>VLRKLKSGLERGLDTFDSTIEIIMQNLKTELESRCSDEVVEQQETENFLEQLISRIFQVVSRLTGVRIRNVQVPDITMEATSENSANVLIPITADVTVSLPFLGEIVDLDLNVDLQTTVSIETDTEDPQVVVGECTNNPESISLTVLHSRFGLVNDVVDIGVNLARRVVSSVVEGELCPRFRELLESLDAECVEKLIGESQ[2x]

Further investigation of BSP30 revealed that it is a mixture of two closely related proteins—BSP30a and BSP30b, sharing 83% amino acid identity, with expression restricted to salivary tissue. Notably, BSP30a and BSP30b are abundantly expressed in the salivary gland independently of one another and the proteins are secreted into saliva, accounting for 15–30% of the total protein in bovine saliva. From a structural point of view, the PLUNC protein family belongs to the TULIP (tubular lipid-binding) superfamily. Each molecule consists of 7 α helices and 6 β strands as well as connecting turns and loops, which constitute the conserved TULIP fold.

We have also solved the structure of BSP30b in complex with oleic acid which shows that the hydrophobic channel can sequester one molecule after co-crystallization. The only structure that revealed elongated stretches of electron density within the hydrophobic tunnel was the complex between BSP30b and oleic acid. The hydrophobic end of oleic acid is buried in the tunnel and its carboxyl group stretches out from the tunnel’s opening, forming hydrogen bonds with the carboxyl group of ASP112 and the carbonyl group of ILE113. We suggest that the hydrophobic tail of oleic acid first “glides” into the internal cavity, driven by multiple hydrophobic interactions, while its carboxyl group stretches out and is stabilised by forming hydrogen bonds with the proximate amino acids. We also observe that the overall structure of BSP30b and its internal cavity remain almost completely unchanged upon binding of the lipid ligand, suggesting that the internal cavity of BSP30b also forms a rigid scaffold for its lipid ligands. Only the helix α3 moves slightly away. One of these sites is occupied to a greater extent than the other and a refinement of the occupancy for the binding site of the dominant ligand showed 80% occupancy for this molecule. From our BSP30b-oleic acid structure, it is obvious that, unlike the changes proposed for SPLUNC1, no major conformational change is needed for lipid binding.Pif1 is a multifunctional helicase and DNA processing enzyme that has roles in genome stability. Pif1 proteins are monomeric enzymes and members of helicase superfamily 1 (SF1), while the 5′–3′ polarity of unwinding place them in the SF1B subgroup. The hPIF1 helicase has the domain architecture characteristic of the SF1B RecD2 helicase subgroup. The overall organization of these domains is similar in all nucleotide bound and free structures determined. hPIF1 has three structural domains, two RecA-like domains 1A (residues 206–381, blue in Figure 1) and 2A (residues 382–435) and domain 2B (residues 436–548, green in Figure 1) with a SRC Homology 3 (SH3)-like fold, in addition to the small functional domain 1B within domain 1A (residues 280–300, cyan in Figure 1).

Here, we describe the first high-resolution crystal structures of hPIF1HD, including an apo structure at 1.44 Å, and a complex with the nucleotide analogue AMP-PNP at 1.13 Å. During ATP binding, represented by the AMP-PNP structure, R381 recognizes the γ-phosphate of ATP. This interaction involves a significant movement of the residue and the 1A–2A inter-domain linker relative to the apo conformation. As such, the aromatic side chain of the adjacent W380 (motif IV) then stacks with the adenine base and together with Y236 forms a pocket for the base. R584 also shifts in position to interact with the ATP γ-phosphate, fixing the α13 helix (domain 2A) relative to the ATP-binding pocket, while Q346 from motif III coordinates the ATP γ-phosphate. Importantly, this conformational rearrangement of the 1A–2A inter-domain linker (W380 and R381) during nucleotide binding causes a significant ∼4 Å shift of the N-terminal end of the α9 helix, which in turn induces a structural rearrangement of the 2B domain. However, a comparison of our 1.13 Å AMP-PNP structure with our 1.44 Å apo structure shows that the binding of the nucleotide induces movement of the Walker A motif (residues 228GSAGTGKS235). Interestingly, the ATP-binding pocket in the 1.13Å human PIF1-AMP-PNP structure more closely resembles that in the yeast Pif1-ADP•ALF4−-ssDNA complex and much of the water structure is conserved (right), while there are substantive movements when the human hPIF1 apo and AMP-PNP structures are compared. Consequently, loop 412–417 becomes more flexible and allows a distortion of the β-sheet β20–β19–β7–β18 and adjustment of its interactions with the hydrophobic core of domain 2A. Comparing the AMP-PNP structure to apo-hPIF1, the observed overall structural changes during ATP binding are small, corresponding to a ∼2.5 Å anti-clockwise shift of the 2A and 2B domains, as depicted in Figure 3A.

> SRMQLSEEQAAVLRAVLKGQSIFFTGSAGTGKSYLLKRILGSLPPTGTVATASTGVAACHIGGTTLHAFAGIGSGQAPLAQCVALAQRPGVRQGWLNCQRLVIDEISMVEADLFDKLEAVARAVRQQNKPFGGIQLIICGDFLQLPPVTKGSQPPRFCFQSKSWKRCVPVTLELTKVWRQADQTFISLLQAVRLGRCSDEVTRQLQATASHKVGRDGIVATRLCTHQDDVALTNERRLQELPGKVHRFEAMDSNPELASTLDAQCPVSQLLQLKLGAQVMLVKNLSVSRGLVNGARGVVVGFEAEGRGLPQVRFLCGVTEVIHADRWTVQATGGQLLSRQQLPLQLAWAMSIHKSQGMTLDCVEISLGRVFASGQAYVALSRARSLQGLRVLDFDPMAVRCDPRVLHFYATLRRGRSL N-{(4S)-4-AMINO-5-[(2-AMINOETHYL)AMINO]PENTYL}-N'-NITROGUANIDINE | C8 H21 N7 O2 | 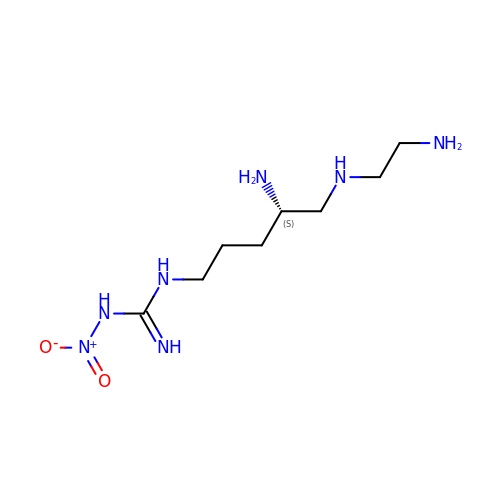RMSWBHUVFNFNIZ-ZETCQYMHSA-N> MFSAGHKIKGTVVLMPKNELEVNPDGSAVD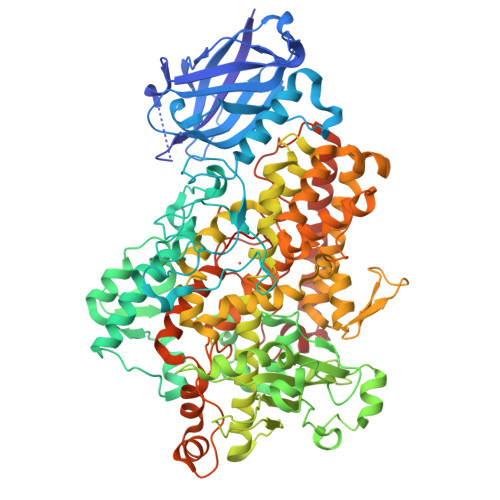NLNAFLGRSVSLQLISATKADAHGKGKVGKDTFLEGINTSLPTLGAGESAFNIHFEWDGSMGIPGAFYIKNYMQVEFFLKSLTLEAISNQGTIRFVCNSWVYNTKLYKSVRIFFANHTYVPSETPAPLVSYREEELKSLRGNGTGERKEYDRIYDYDVYNDLGNPDKSEKLARPVLGGSSTFPYPRRGRTGRGPTVTDPNTEKQGEVFYVPRDENLGHLKSKDALEIGTKSLSQIVQPAFESAFDLKSTPIEFHSFQDVHDLYEGGIKLPRDVISTIIPLPVIKELYRTDGQHILKFPQPHVVQVSQSAWMTDEEFAREMIAGVNPCVIRGLEEFPPKSNLDPAIYGDQSSKITADSLDLDGYTMDEALGSRRLFMLDYHDIFMPYVRQINQLNSAKTYATRTILFLREDGTLKPVAIELSLPHSAGDLSAAVSQVVLPAKEGVESTIWLLAKAYVIVNDSCYHALMSHWLNTHAAMEPFVIATHRHLSVLHPIYKLLTPHYRNNMNINALARQSLINANGIIETTFLPSKYSVEMSSAVYKNWVFTDQALPADLIKRGVAIKDPSTPHGVRLLIEDYPYAADGLEIWAAIKTWVQEYVPLYYARDDDVKNDSELQHWWKEAVEKGHGDLKDKPWWPKLQTLEDLVEVCLIIIWIASALHAAVNFGQYPYGGLIMNRPTASRRLLPEKGTPEYEEMINNHEKAYLRTITSKLPTLISLSVIEILSTHASDEVYLGQRDNPHWTSDSKALQAFQKFGNKLKEIEEKLVRRNNDPSLQGNRLGPVQLPYTLLYPSSEEGLTFRGIPNSISI>PPERGGAGTSQDGTSKNCFKITIPYGRKYDKAWLLSMIQSKCSVPFTPIEFHYENTRAQFFVEDASTASALKAVNYKILDRENRRISIIINSSAPPHTILNELKPEQVEQLKLIMSKRYDGSQQVLDLKGLRSDPDLV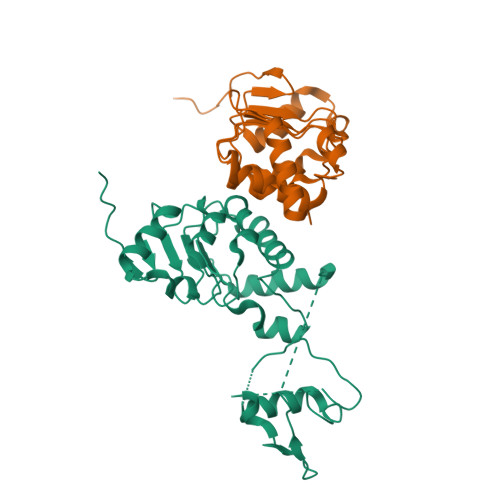AQNIDVVLNRRSCMAATLRIIEENIPELLSLNLSNNRLYRLDDMSSIVQKAPNLKILNLSGNELKSERELDKIKGLKLEELWLDGNSLCDTFRDQSTYISAIRERFPKLLRLDGHELPPPIAFDVEAPTTLPP[2x]> ETPPRFTRTPVDQTGVSGGVASFICQATGDPRPKIVWNKKGKKVSNQRFEVIEFDDGSGSVLRIQPLRTPRDEAIYECVASNNVGEISVSTRLTVLREDQIPRGFPTIDMGPQLKVVERTRTATMLCAASGNPDPEITWFKDFLPVDTSNNNGRIKQLRSESIGGTPIRGALQIEQSEESDQGKYECVATNSAGTRYSAPANLYVRELREVRRVPPRFSIPPTNHEIMPGGSVNITCVAVGSPMPYVKWMLGAEDLTPEDDMPIGRNVLELNDVRQSANYTCVAMSTLGVIEAIAQITVKALPKPPGTPVVTESTATSITLTWDSGNPEPVSYYIIQHKPKNSEEPYKEIDGIATTRYSVAGLSPYSDYEFRVVAVNNIGRGPASEPVLTQTSEQAPSSAPRDVQARMLSSTTILVQWKEPEEPNGQIQGYRVYYTMDPTQHVNNWMKHNVADSQITTIGNLVPQKTYSVKVLAFTSIGDGPLSSDIQVITQTGVPGQPLNFKAEPESETSILLSWTPPRSDTIASYELVYRDGDQGEEQRITIEPGTSYRLQGLKPNSLYYFRLSARSPQGLGASTAEISARTMQSMFAKNFHVKAVMKTSVLLSWEIPENYNSAMPFKILYDDGKMVEEVDGRATQKLIVNLKPEKSYSFVLTNRGNSAGGLQHRVTAKTAPDVLRTKPAFIGKTNLDGMITVQLPDVPANENIKGYYIIIVPLKKSRGKFIKPWESPDEMELDELLK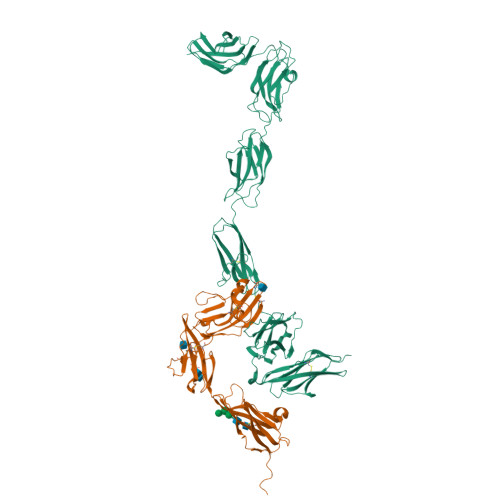EISRKRRSIRYGREVELKPYIAAHFDVLPTEFTLGDDKHYGGFTNKQLQSGQEYVFFVLAVMDHAESKMYATSPYSDPVVSMDLDPQPITDEEEKHHHHHH;> AQPAARDLKVVTKRGSADGCTDWSVDIKKYQVLVGEPVRIKCALFYGYIRTNYSLAQSAGLSLMWYKSSGPGDFEEPIAFDGSRMSKEEDSIWFRPTLLQDSGLYACVIRNSTYCMKVSISLTVGENDTGLCYNSKMKYFEKAELSKSKEISCRDIEDFLLPTREPEILWYKECRTKAWRPSIVFKRDTLLIKEVKEDDIGNYTCELKYGGFVVRRTTELTVTAPLTDKPPKLLYPMESKLTVQETQLGGSANLTCRAFFGYSGDVSPLIYWMKGEKFIEDLDENRVWESDIRILKEHLGEQEVSISLIVDSVEEGDLGNYSCYVENGNGRRHASVLLHKRKHHHHHH>[2x]MASSNLIKQLQERGLVAQVTDEEALAERLAQGPIALYCGFDPTADSLHLGHLVPLLCLKRFQQAGHKPVAVVGGATGLIGDPSFKAAERKLNTEETVQEWVDKIRKQVAPFLDFDCGENSAIAANNYDFFGNMNVLTFLRDIGKHFSVNQMINKEAVKQRLNREDQGISFTEFSYNLLQGYGFACLNKQYGVVLQIGGSDQWGNITSGIDLTRRLHQNQVFGLTVPLITKADGTKFGKTEGGA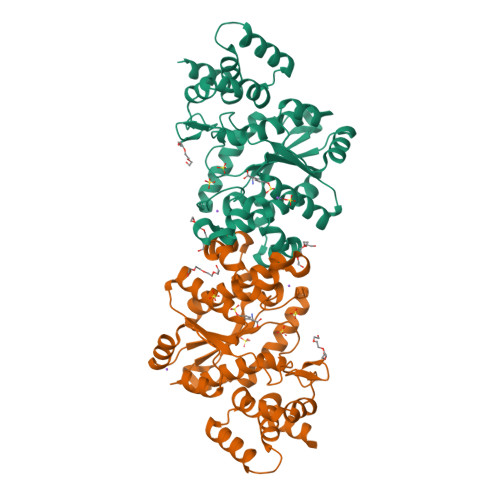VWLDPKKTSPYKFYQFWINTADADVYRFLKFFTFMSIEEINALEEEDKNSGKAPRAQYVLAEQVTRLVHGEEGLQAAKR> QCDVPPNSRFDCAPDKAITQEQCEARGCCYIPAKQGLQGAQMGQPWCFFPPSYPSYKLENLSSSEMGYTATLTRTTPTFFPKDILTLRLDVMMETENRLHFTIKDPANRRYEVPLETPRVHSRAPSPLYSVEFSEEPFGVIVHRQLDGRVLLNTTVAPLFFADQFLQLSTSLPSQYITGLAEHLSPLMLSTSWTRITLWNRDLAPTPGANLYGSHPFYLALEDGGSAHGVFLLNSNAMDVVLQPSPALSWRSTGGILDVYIFLGPEPKSVVQQYLDVVGYPFMPPYWGLGFHLCRWGYSSTAITRQVVENMTRAHFPLDVQWNDLDYMDSRRDFTFNKDGFRDFPAMVQELHQGGRRYMMIVDPAISSSGPAGSYRPYDEGLRRGVFITNETGQPLIGKVWPGSTAFPDFTNPTALAWWEDMVAEFHDQVPFDGMWIDMNEPSNFIRGSEDGCPNNELENPPYVPGVVGGTLQAATICASSHQFLSTHYNLHNLYGLTEAIASHRALVKARGTRPFVISRSTFAGHGRYAGHWTGDVWSSWEQLASSVPEILQFNLLGVPLVGADVCGFLGNTSEELCVRWTQLGAFYPFMRNHNSLLSLPQEPYSFSEPAQQAMRKALTLRYALLPHLYTLFHQAHVAGETVARPLFLEFPKDSSTWTVDHQLLWGEALLITPVLQAGKAEVTGYFPLGTWYDLQTVPIEALGSLPPPPAAPREPAIHSEGQWVTLPAPLDTINVHLRAGYIIPLQGPGLTTTESRQQPMALAVALTKGGEARGELFWDDGESLEVLERGAYTQVIFLARNNTIVNELVRVTSEGAGLQLQKVTVLGVATAPQQVLSNGVPVSNFTYSPDTKVLD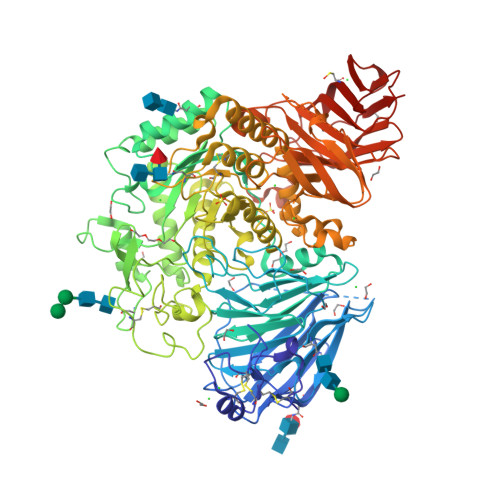ICVSLLMGEQFLVSWC>[4x]MTIMLTPMQTEEFRSYLTYTTKHYAEEKVKAGTWLPEDAQLLSKQVFTDLLPRGLE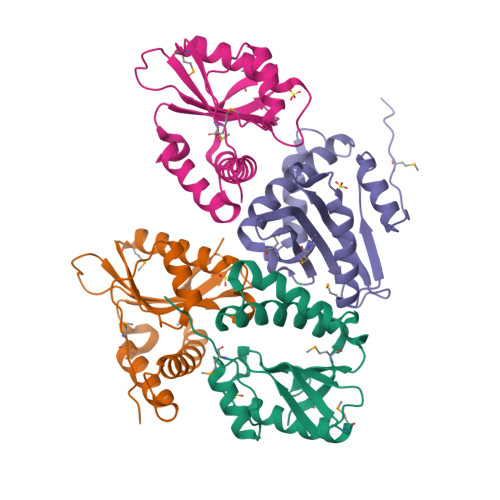TPHHHLWSLKLNEKDIVGWLWIHAEPEHPQQEAFIYDFGLYEPYRGKGYAKQALAALDQAARSMGIRKLSLHVFAHNQTARKLYEQTGFQETDVVMSKKLLE> MGNCHTVGPNEALVVSGGCCGSDYKQYVFGGWAWAWWCISDTQRLSLEVMTILCRCENIETSEGVPLFVTGVAQVKIMTEKELLAVACEQFLGKNVQDIKNVVLQTLEGHLRSILGTLTVEQIYQDRDQFAKLVREVAAPDVGRMGIEILSFTIKDVYDKVDYLSSLGKTQTAVVQRDADIGVAEAERDAGIREAECKKEMLDVKFMADTKIADSKRAFELQKSAFSEEVNIKTAEAQLAYELQGAREQQKIRQEEIEIEVVQRKKQIAVEAQEILRTDKELIATVRRPAEAEAHRIQQIAEGEKVKQVLLAQAEAEKIRKIGEAEAAVIEAMGKAEAERMKLKAEAYQKYGDAAKMALVLEALPQIAAKIAAPLTKVDEIVVLSGDNSKVTSEVNRLLAEL;> MFFTCGPNEAMVVSGFCRSPPVMVAGGRVFVLPCIQQIQRISLNTLTLNVKSEKVYTRHGVPISVTGIAQVKIQGQNKEMLAAACQMFLGKTEAEIAHIALETLEGHQRAIMAHMTVEEIYKDRQKFSEQVFKVASSDLVN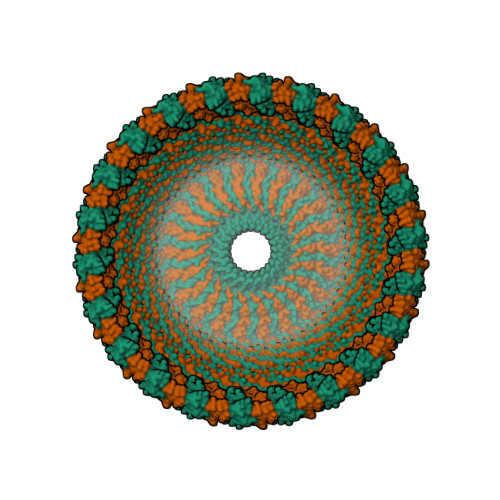MGISVVSYTLKDIHDDQDYLHSLGKARTAQVQKDARIGEAEAKRDAGIREAKAKQEKVSAQYLSEIEMAKAQRDYELKKAAYDIEVNTRRAQADLAYQLQVAKTKQQIEEQRVQVQVVERAQQVAVQEQEIARREKELEARVRKPAEAERYKLERLAEAEKSQLIMQAEAEAASVRMRGEAEAFAIGARARAEAEQMAKKAEAFQLYQEAAQLDMLLEKLPQVAEEISGPLTSANKITLVSSGSGTMGAAKVTGEVLDILTRLPESVERLTGVSISQVNHK>MNTVSPAKKKVIII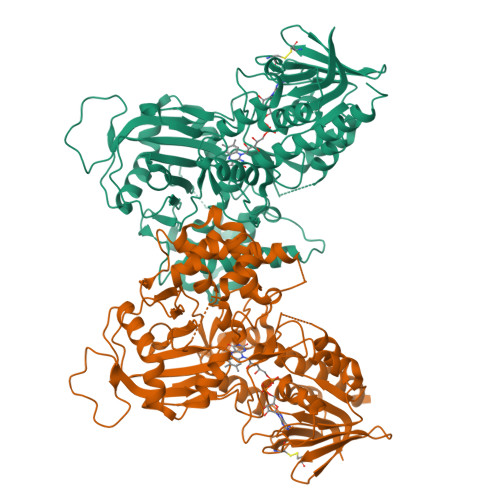GAGIAGLKAASTLHQNGIQDCLVLEARDRVGGRLQTVTGYQGRKYDIGASWHHDTLTNPLFLEEAQLSLNDGRTRFVFDDDNFIYIDEERGRVDHDKELLLEIVDNEMSKFAELEFHQHLGVSDCSFFQLVMKYLLQRRQFLTNDQIRYLPQLCRYLELWHGLDWKLLSAKDTYFGHQGRNAFALNYDSVVQRIAQSFPQNWLKLSCEVKSITREPSKNVTVNCEDGTVYNADYVIITVPQSVLNLSVQPEKNLRGRIEFQPPLKPVIQDAFDKIHFGALGKVIFEFEECCWSNESSKIVTLANSTNEFVEIVRNAENLDELDSMLEREDSQKHTSVTCWSQPLFFVNLSKSTGVASFMMLMQAPLTNHIESIREDKERLFSFFQPVLNKIMKCLDSEDVIDGMRPIENIANANKPVLRNIIVSNWTRDPYSRGAYSACFPGDDPVDMVVAMSNGQDSRIRFAGEHTIMDGAGCAYGAWESGRREATRISDLLKLEHHH[2x]> MSLTTVGIRGTFFDFVDDPWKHIGNEQAAARFHQDGLMVVTDGVIKAFGPYEKIAAAHPGVEITHI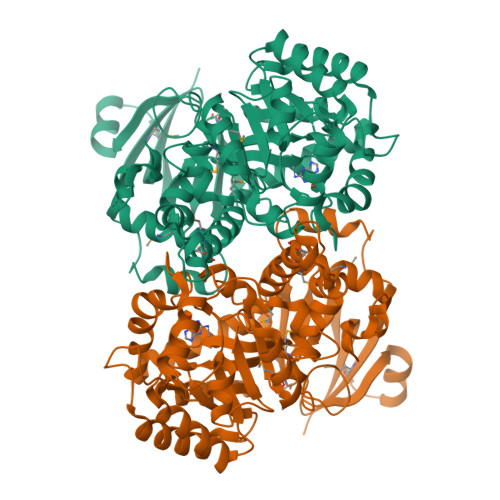KDRIIVPGFIDGHIHLPQTRVLGAYGEQLLPWLQKSIYPEEIKYKDRNYAREGVKRFLDALLAAGTTTCQAFTSSSPVATEELFEEASRRNMRVIAGLTGIDRNAPAEFIDTPENFYRDSKRLIAQYHDKGRNLYAITPRFAFGASPELLKACQRLKHEHPDCWVNTHISENPAECSGVLVEHPDCQDYLGVYEKFDLVGPKFSGGHGVYLSNNEFRRMSKKGAAVVFCPCSNLFLGSGLFRLGRATDPEHRVKMSFGTDVGGGNRFSMISVLDDAYKVGMCNNTLLDGSIDPSRKDLAEAERNKLSPYRGFWSVTLGGAEGLYIDDKLGNFEPGKEADFVALDPNGGQLAQPWHQSLIADGAGPRTVDEAASMLFAVMMVGDDRCVDETWVMGKRLYKKSEGHHHHHH> TELTLKPGTLTLAQLRAIHAAPVRLQLDASAAPAIDASVACVEQIIAEDRTAYGINTGFGLLASTRIASHDLENLQRSLVLSHAAGIGAPLDDDLVRLIMVLKINSLSRGFSGIRRKVIDALIALVNAEVYPHIPLKGSVGASGDLAPLAHMSLVLLGEGKARYKGQWLSATEALAVAGLEPLTLAAKEGLALLNGTQASTAYALRGLFYAEDLYAAAIACGGLSVEAVLGSRSPFDARIHEARGQRGQIDTAACFRDLLGDSSEVSLSHKNADKVQDPYSLRCQPQVMGACLTQLRQAAEVLGIEANAVSDNPLVFAAEGDVISGGNFHAEPVAMAADNLALAIAEIGSLSERRISLMMDKHMSQLPPFLVENGGVNSGFMIAQVTAAALASENKALSHPHSVDSLPTSANQEDHVSMAPAAGKRLWEMAENTRGVL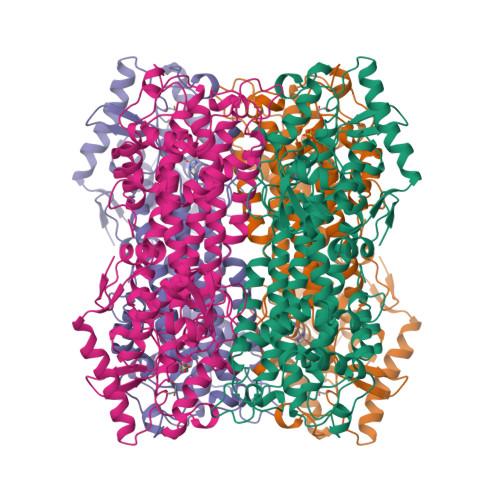AIEWLGACQGLDLRKGLKTSAKLEKARQALRSEVAHYDRDRFFAPDIEKAVELLAKGSLTGLLPAGVLPSL>[2x]METKWRNGDIVQPVLNPEPNTVSYSQSSLIHLVGP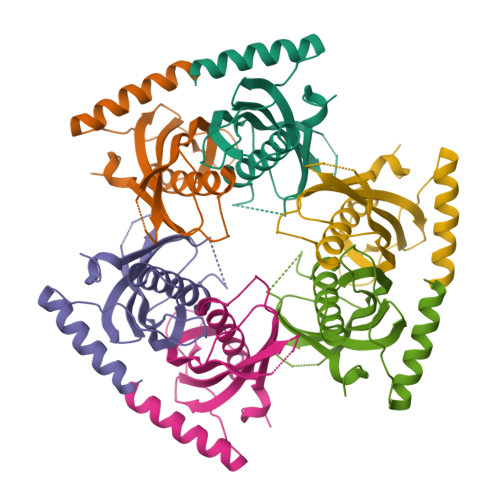SDCTLHGFVHGGVTMKLMDEVAGIVAARHCKTNIVTASVDAINFHDKIRKGCVITISGRMTFTSNKSMEIEVLVDADPVVDNSQKRYRAASAFFTYVSLNQEGKPMPVPQLVPETEDEKKRFEEGKGRYLQMKAKRQGHTEPQP>MLDIKLIRENPELVKNDLIKRGELEKVKWVDEILKLDTEWRTKLKEINRLRHERNKIAVEIGKRRKKGEPVDELLAKSREIVKRIGELENEVEELKKKIDYYLWRLPNITHPSVPVGKDENDNVPIRFWGKARVWKGHLERFLEQSQGKMEYEILEWKPKLHVDLLEILGGADFARAAKVSGSRFYYLLNEIVILDLALIRFALDRLIEKGFTPVIPPYMVRRFVEEGSTSFEDFEDVIYKVEDEDLYLIPTAEHPLAGMHANEILDGKDLPLLYVGVSPCFRKEAGTAGKDTKGIFRVHQFHKVEQFVYSRPEESWEWHEKIIRNAEELFQELEIPYRVVNICTGDLGYVAAKKYDIEAWMPGQGKFREVVSASNCTDWQARRLNIRFRDRTDEKPRYVHTLNSTAIATSRAIVAILENHQE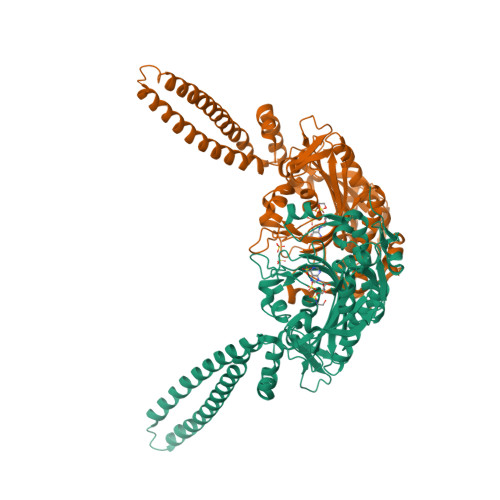EDGTVRIPKVLWKYTGFKEIVPVEKKERCCAT[2x]> MEFFGESWKKHLSGEFGKPYFIKLMGFVAEERKHYTVYPPPHQVFTWT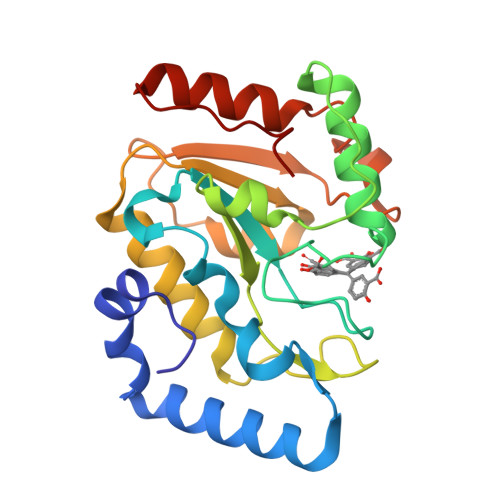QMCDIKDVKVVILGQDPYHGPNQAHGLCFSVQRPVPPPPSLENIYKELSTDIEDFVHPGHGDLSGWAKQGVLLLNAVLTVRAHQANSHKERGWEQFTDAVVSWLNQNSNGLVFLLWGSYAQKKGSAIDRKRHHVLQTAHPSPLSVYRGFFGCRHFSKTNELLQKSGKKPIDWKEL>GPKEVYLDRKLLTLEDKELGSGNFGTVKKGYYQMKKVVKTVAVKILKNEANDPALKDELLAEANVMQQLDNPYIVRMIGICEAESWMLVMEMAELGPLNKYLQQNRHVKDKNIIELVHQVSMGMKYLEESNFVHRDLAARNVLLVTQHYAK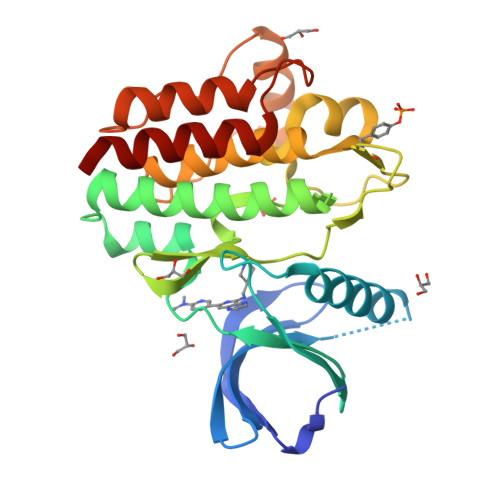ISDFGLSKALRADENYYKAQTHGKWPVKWYAPECINYYKFSSKSDVWSFGVLMWEAFSYGQKPYRGMKGSEVTAMLEKGERMGCPAGCPREMYDLMNLCWTYDVENRPGFAAVELRLRNYYYDVVN[2x]>MSLDQIKIAYIGGGSQGWARSLMSDLSIDERMSGTVALYDLDFEAAQKNEVIGNHSGNGRWRYEAVSTLKKALSAADIVIISILPGSLDDMEVDVHLPERCGIYQSVGDTVGPGGIIRGLRAVPIFAEIARAIRDYAPESWVINYTNPMSVCTRVLYKVFPGIKAIGCCHEVFGTQKLLAEMVTERLGIEVPRREDIRVNVLGINHFTWITKASYRHIDLLPIFREFSAHYGESGYELEGECWRDSVFCSAHRVAFDLFETYGAIPAAGDRHLAEFLPGPYLKQPEVWKFHLTPISFRKQDRAEKRQETERLIVQQRGVAEKASGEEGVNIIAALLGLGELVTNVNMPNQGQVLNLPIQAIVETNAFITRNRVQPILSGALPK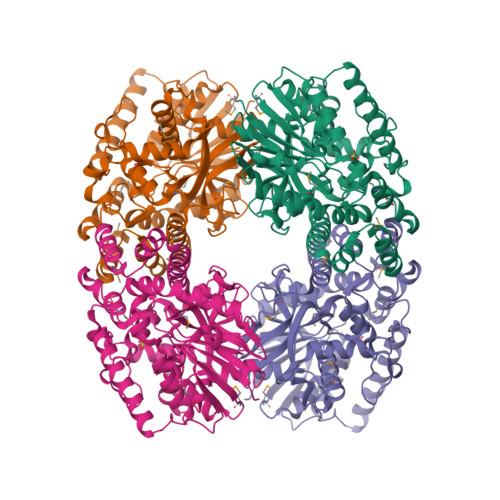GVEMLAARHISNQEAVADAGLTKDTGLAFQAFLNDPLVQIDRSDAEQLFNDMLQCIMQSEGHHHHHH[4x]>MHHHHHHDYKDDDDKAPVQAADEMYDSNPHPDRRQLVSNGFEVNLPDQVEVIVRDLPDPSKVKEERTRLMGYWFVHWFDGKLFHLRIKAGGPNVDGEHRAIRTAEHPWLLRARLDDALEEALPKYAAVKKRPFTFLAQKDELIDAAATAAGLSHRLLNSFKVIPRFALSPKIYEPVDGTTRVGVFVTIGMRYDIEASLRDLLEAGIDLRGMYVVRRKRQPGERGLLGRVRAISDDMVQLFEETDLASVNVNDAKLEGSKENFTRCLSALLGHNYKKLLNALDDQEAGYRTGPRFDDAVRRMGEFLAKKPIRLADNINAQVGDRIVFSNEGQARNVRLAPKVEYVFDRTGAKSAEYAWRGLSQFGPFDRPSFANRSPRILVVYPSSTQGKVENFLSAFRDGMGSNYSGFSKGFVDLMGLTKVEFVMCPVEVSSADRNGAHTKYNSAIEDKLAGAGEVHAGIVVLFEDHARLPDDRNPYIHTKSLLLTLGVPTQQVRMPTVLLEPKSLQYTLQNFSIATYAKLNGTPWTVNHDKAINDELVVGMGLAELSGSRTEKRQRFVGITTVFAGDGSYLLGNVSKECEYEGYSDAIRESMTGILRELKKRNNWRPGDTVRVVFHAHRPLKRVDVASIVFECTREIGSDQNIQMAFVTVSHDHPFVLIDRSERGLEAYKGSTARKGVFAPPRGAISRVGRLTRLLAVNSPQLIKR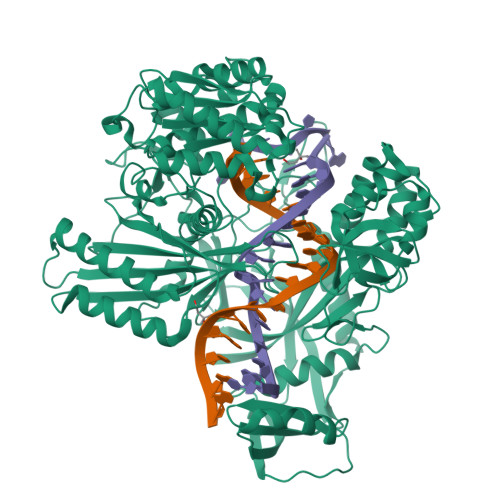ANTPLPTPLLVSLHPDSTFKDVDYLAEQALKFTSLSWRSTLPAATPVTIFYSERIAELLGRLKSIPNWSSANLNIKLKWSRWFL[2x]>MVDSRNADTEQENENLSKFCIDMTAMAREGKIDPVIGREEEIRRVIRILSRRTKNNPVLIGEPGVGKTTIVEGLAQRIVNADVPDNLAACKLLSLDVGALVAGSKYRGEFEERMKGVLKEIQESKETIILFVDEIHLLMGAGSSGEGGMDAANLLKPMLARGQLHCIGATTLAEYRKYIEKDAAFERRFQQVLVKEPSITETISILRGLKEKYEVHHGVNIADAAIVAAANLAARYLTSRRLPDSAVDLIDEAAAAVRVARESQPEIIDSLERRLRQLKIEIHALSREKDEASKARLAQAKQDAQNVEEELRPLREKYERERQRGKAIQEAKMKLEALRVKAEDASRMGDHSRAADLQYYAIPEQEAIIKRLEAEKAAADAALNANGADVGGSMITDVVGPDQINEIVARWTGIPVTRLKTSEKEKLLHMEQALSKIVVGQKEAVQSVSNAIRLQRSGLSNPNQPPSFLFCGPSGTGKTLLTKALAEFLFDDPKSMIRFDMSEYQERHSLSRMIGAPPGYVGHDAGGQLTEALRRRPFSILLFDEVEKAAKEVLTVLLQLMDDGRITDGQGRVVDAKNCIVVMTSNLGAEYLSRANNGKDGKIDPTTRELVMNTLRNYFLPEFLNRISSIVIFNRLTRREIRKIVDLRIAEIQKRLTDNDRNVTIKVSDEAKDKLGAQGYSPVYGARPLQRLLEKEVLNRLAILILRGQIREGEVACVELVDGKVQVLPNHPDSEPEDVDVD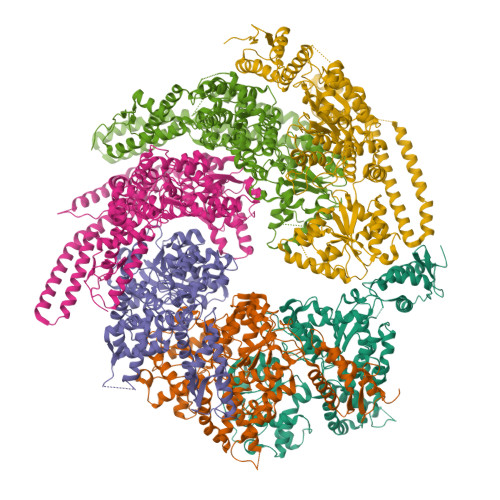MESDDAVDEVAPDSMDEDIYND[6x]> EEEE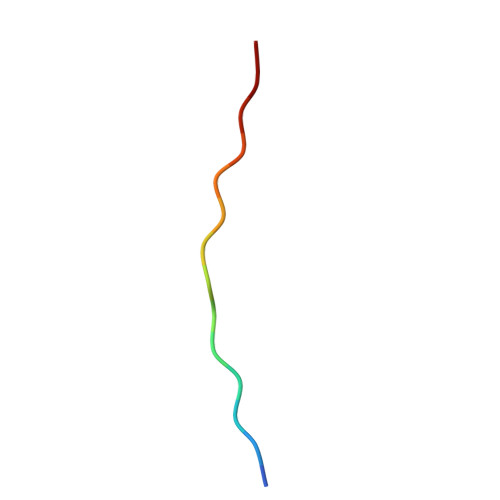EEEEEEEEEE> MATLFIADLHLCVAAPAITAGFLRFLAGEARKADAL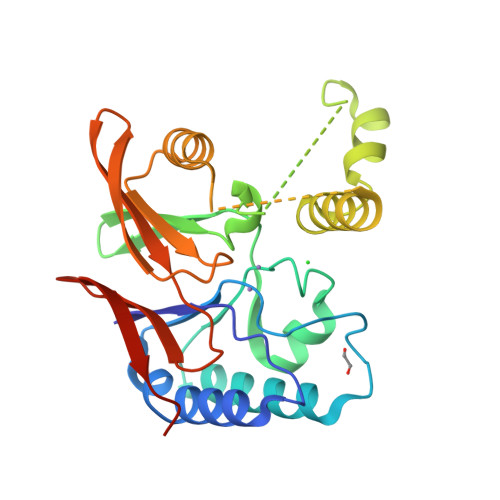YILGDLFEAWIGDDDPNPLHRKMAAAIKAVSDSGVPCYFIHGNRDFLLGKRFARESGMTLLPEEKVLELYGRRVLIMHGDTLCTDDAGYQAFRAKVHKPWLQTLHSALPSHVRKRIAARMRANSTAANSSKSLAIMDVNQNAVVSAMEKHQVQWLIHGHTHRPAVHELIANQQPAFRVVLGAWHTEGSMVKVTADDVELIHFPFLEHHHHHH>[4x]MAAGSITTLPALPEDG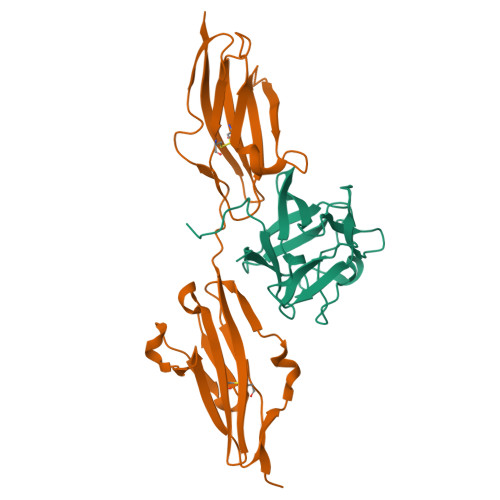GSGAFPPGHFKDPKRLYCKNGGFFLRIHPDGRVDGVREKSDPHIKLQLQAEERGVVSIKGVSANRYLAMKEDGRLLASKSVTDECFFFERLESNNYNTYRSRKYTSWYVALKRTGQYKLGSKTGPGQKAILFLPMSAKS;>NSNNKRAPYWTNTEKMEKRLHAVPAANTVKFRCPAGGNPMPTMRWLKNGKEFKQEHRIGGYKVRNQHWSLIMESVVPSDKGNYTCVVENEYGSINHTYHLDVVERWPHRPILQAGLPANASTVVGGDVEFVCKVYSDAQPHIQWIKHVEKNGSKYGPDGLPYLKVLKAAGVNTTDKEIEVLYIRNVTFEDAGEYTCLAGNSIGISFHSAWLTVLPAPGRE[4x]>ETGSAQQLNEDLRLHLLLNTSVTCNDGSPAGYYLKESRGSRRWLLFLEGGWYCFNRENCDSRYDTMRRLMSSRDWPRTRTGTGILSSQPEENPYWWNANMVFIPYCSSDVWSGASSKSEKNEYAFMGALIIQEVVRELLGRGLSGAKVLLLAGSAAGGTGVLLNVDRVAEQLEKLGYPAIQVRGLADSGWFLDNKQYRHTDCVDTITCAPTEAIRRGIRYWNGVVPERCRRQFQEGEEWNCFFGYKVYPTLRSPVFVVQWLFDEAQLTVDNVHLTGQPVQEGLRLYIQNLGRELRHTLKDVPASFAPACLSHEIIIRSHWTDVQVKGTSLPRALHCWDRSLHDSHKASKTPLKGCPVHLVDSCPWPHCNPSCPTGTKHHHHHH[2x]

We recently identified the Wnt antagonist Notum, a member of the α/β hydrolase superfamily, as a Wnt deacylase that can remove large (C16) palmitoleate lipids from Wnt ligands. Importantly, Wnt acylation is reversible upon the activity of Notum, a secreted carboxylesterase that acts as a feedback inhibitor of Wnt signalling. Stomach-produced ghrelin is a 28 amino acid-secreted peptide with an eight carbon fatty acid covalently linked to the side chain oxygen atom of the third serine residue. We have provided biochemical and structural evidence showing that the Wnt-deacylating enzyme Notum can also deacylate ghrelin.

We determined the crystal structure, which showed at high resolution how this enzyme engages with the octanoyl lipid substrate. To the best of our knowledge, this is the first reported structure of ghrelin with a cognate deacylase. The interactions between the ghrelin octanoyl lipid and Notum were mainly hydrophobic. The lipid tail interacted with I291, F268, F320, and Y129, while the lipid head interacted with G127, W128, A233, and H389. Hydrogen bonds formed between the octanoyl acid and the backbones of G127, W128, and A233 and the side chain of H389. Compared with the apo Notum structure, all of the interacting residues maintained their side chain conformations, except Y129. The Y129 was repositioned to interact with the octanoyl lipid in the ghrelin complex with (the closest side chain carbon) distances of 3.6 and 3.7 Å to C4 and C5 of the lipid, respectively (for the superimposed apo structure, the equivalent distances were 4.7 and 4.5 Å, respectively). When the peptide was treated with active Notum enzyme, the m/z shifted to 3511.84 with a double-charged peak of 1756.92. The loss of 126.13 Da matched well with an 8-carbon chain, indicating complete removal of the octanoyl lipids. In contrast, when the inactive Notum mutant (S232A) enzyme was used, the mass of the untreated peptide was retained.>GHMSTLLINQPQYAWLKELGLREENEGVYNGSWGGRGEVITTYCPANNEPIARVRQASVADYEETVKKAREAWKIWADIPAPKRGEIVRQIGDALREKIQVLGSLVSLEMGKILVEGVGEVQEYVDICDYAVGLSRMIGGPILPSERSGHALIEQWNPVGLVGIITAFNFSVAVYGWNNAIAMICGNVCLWKGAPTTSLISVAVTKIIAKVLEDNKLPGAICSLTCGGADIGTAMAKDERVNLLSFTGSTQVGKQVGLMVQERFGRSLLELGGNNAIIAFEDADLSLVVPSALFAAVGTAGQRCTTARRLFIHESIHDEVVNRLKKAYAQIRVGNPWDPNVLYGPLHTKQAVSMFLGAVEEAKKEGGTVVYGGKVMDRPGNYVEPTIVTGLGHDASIAHTETFAPILYVFKFKNEEEVFAWNNEVKQGLSSSIFTKDLGRIFRWLGPKGSDCGIVNVNIPTSGAEIGGAFGGEKHTGG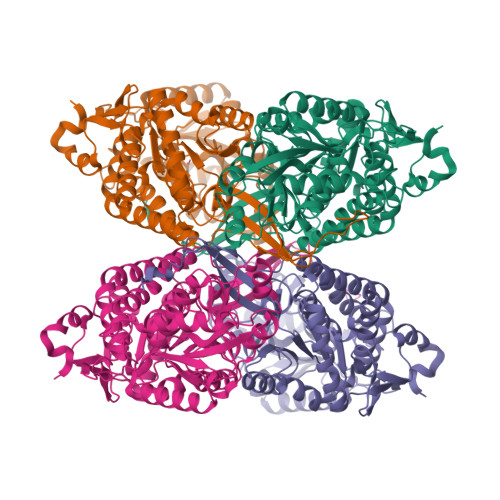GRESGSDAWKQYMRRSTCTINYSKDLPLAQGIKFQ[8x]>GQDSTSDLIPAPPLSKVPLQQNFQDNQFQGKWYVVGLAGNAILREDKDPQKMYATIYELKEDKSYNVTSVLFRKKKCDYWIRTFVPGSQPGEFTLGNIKSYPGLTSYLVRVVSTNYNQHAMV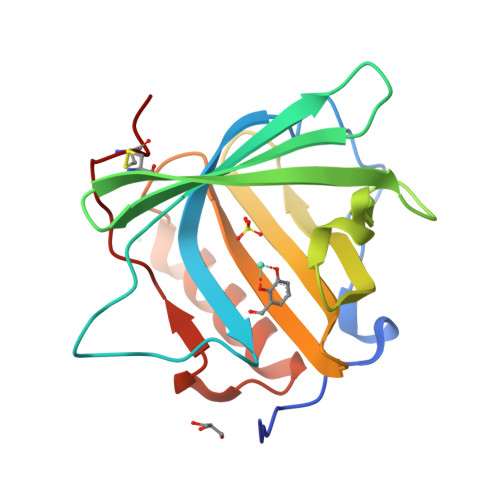FFKKVSQNREYFKITLYGRTKELTSELKENFIRFSKSLGLPENHIVFPVPIDQCIDG[3x]Here, we report substrate‐bound crystal structures and rational engineering of substrate and stereo‐specificities of UGT85B1 from Sorghum bicolor involved in biosynthesis of the cyanogenic glucoside dhurrin. Finally, (S)‐p‐hydroxymandelonitrile is stabilized by glucosylation catalyzed by SbUGT85B1, resulting in the formation of dhurrin (Jones et al., 1999). UGTs are a superfamily of enzymes that use UDP‐activated sugar donors to transfer a sugar moiety to an acceptor molecule. The structures reveal the characteristic UDP‐glycosyltransferase GT‐B fold found in all known plant UGTs (Lairson et al., 2008) with two Rossman domains forming a narrow catalytic cleft, where the N‐terminal domain predominantly interacts with p‐hydroxymandelonitrile, while the C‐terminal domain predominantly interacts with UDP.

The UDP binding site is characterized by the presence of the highly conserved family‐defining Plant Secondary Product Glycosyltransferase (PSPG) motif (Osmani et al., 2009), and consists of residues W368, C369, Q371, H386, N390, S391, E394, and Q411, as well as residues Q21, E288, N308, S311, and V337. Coordination of S391 with the pyrophosphate group confirms a previous hypothesis of S391 to stabilize binding of UDP‐glucose (Thorsøe et al., 2005). In contrast, R201, also previously hypothesized to stabilize binding of UDP‐glucose (Thorsøe et al., 2005), is not in the active site, and is located 22 Å from UDP. The binding mode of UDP in the sugar donor active site is identical in the two structures, and thus not affected by the presence of p‐hydroxymandelonitrile in the sugar acceptor binding site. The two structures are highly similar (root mean square deviation [RMSD] = 0.17 Å over all 6148 atoms), thus not indicating significant structural changes upon binding of p‐hydroxymandelonitrile. Crystals were developed by the sitting drop method and the structure was solved via molecular replacement using MtUGT85H2 (Li et al., 2007). Finally, the high resolution of the UDP–sugar binding site may enable engineering of sugar donor preference for the production of new‐to‐nature compounds with tailored properties.

> MGSNAPPPPTPHVVLVPFPGQGHVAPLMQLARLLHARGARVTFVYTQYNYRRLLRAKGEAAVRPPATSSARFRIEVIDDGLSLSVPQNDVGGLVDSLRKNCLHPFRALLRRLGQEVEGQDAPPVTCVVGDVVMTFAAAAAREAGIPEVQFFTASACGLLGYLHYGELVERGLVPFRDASLLADDDYLDTPLEWVPGMSHMRLRDMPTFCRTTDPDDVMVSATLQQMESAAGSKALILNTLYELEKDVVDALAAFFPPIYTVGPLAEVIASSDSASAGLAAMDISIWQEDTRCLSWLDGKPAGSVVYVNFGSMAVMTAAQAREFALGLASCGSPFLWVKRPDVVEGEEVLLPEALLDEVARGRGLVVPWCPQAAVLKHAAVGLFVSHCGWNSLLEATAAGQPVLAWPCHGEQTTNCRQLCEVWGNGAQLPREVESGAVARLVREMMVGDLGKEKRAKAAEWKAAAEAAARKGGASWRNVERVVNDLLLVGGKQHHHHHH4-(dihydroxyboranyl)-2-({[4-(phenylsulfonyl)thiophen-2-yl]sulfonyl}amino)benzoic 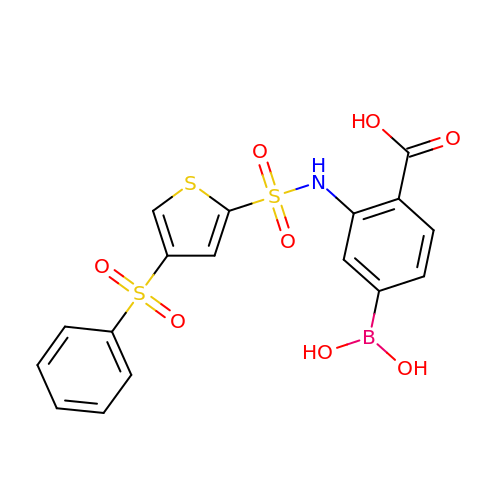acid | C17 H14 B N O8 S3 | JJPKFZAOXOEFHQ-UHFFFAOYSA-N>[2x]GPAAKSPENVYPVKTFGFAAKDSSGFFSPFNFSRRATGENDVQFKVLYCGTCNYDLEMSTNKFGMTKYPFVIGHEIVGVVTEIGSKVQKFKVGDKVGVGGFVGACEKCEMCVNGVENNCSKVESTDGHFGNNFGGCCNIMVVNEKYAVVWPENLPLHSGVPLLCAGITTYSPLRRYGLDKPGLNIGIAGLGGLGHLAIRFAKAFGAKVTLISSSVKKKREALEKFGVDSFLLNSNPEEMQGAYGTLDGIIDTMPVAHSIVPFLALLKPLGKLIILGVPEEPFEVPAPALLMGGKLIAGSAAGSMKETQEMIDFAAKHNIVADVEVIPIDYLNTAMERIKNSDVKYRFVIDVGNTLKSPSF

Crystal structures of THAS (here referred to as THAS1), a second representative THAS (Cr_021691, THAS2) and the structure of the promiscuous homologue (Cr_032583b, HYS) were solved and mutants revealed key residues that control the stereochemistry of the product profiles. The HYSs perform a single, chemically straightforward reduction reaction that immediately neutralizes the reactivity of strictosidine aglycone/cathenamine. The biological unit is an elongated homodimer, with each subunit divided into a substrate and cofactor-binding domain; the latter also being responsible for forming the dimer interface. The active site cavities of the HYSs are framed by helix α2, the catalytic zinc coordination sphere, and loops 1 and 2, with the NADP(H) co-substrate binding at the base of the active site.

Notably, one enzyme (Cr_032583b, HYS) produced a dramatically different product profile consisting of a mixture of ajmalicine/tetrahydroalstonine/mayumbine (55:27:15, at pH 6). HYS, which has a distinctly different product profile, was also crystallized to explore the structural basis behind this distinct stereochemical outcome. Structures were obtained for THAS1 and THAS2 with NADP+ bound (THAS1, 1.05 Å resolution; THAS2, 2.10 Å resolution) and in apo form (THAS1, 2.25 Å resolution; THAS2, 2.05 Å resolution), while HYS could only be crystallized in the apo form (2.25 Å resolution). The histidine residue in HYS loop 2 (His127) appears to be positioned appropriately to provide an alternative proton source for the opposite (‘top') face of the substrate, which could explain the appearance of ajmalicine in the product profile of HYS. Reactions with THAS1 and HYS performed at different pH conditions revealed that while changes in pH did not substantially impact the product profile of THAS1, HYS produced increased amounts of ajmalicine relative to tetrahydroalstonine at pH 6 compared with higher pH values. The increased level of ajmalicine in HYS at lower pH values is consistent with the pKa value of the histidine side chain and supports the role of this histidine in ajmalicine biosynthesis, though attributing pH dependence to specific residues must be approached with caution. While the THAS1 mutant containing the swaps displayed reduced activity rather than an altered product profile, the HYS mutant containing the shorter THAS1 loop 2 resulted in a product profile similar to that of THAS1. Therefore, we mutated this histidine to alanine or asparagine in HYS. Both of these mutants gave the same THAS-like profile, suggesting that His127 is required for producing the ajmalicine (R C20) stereochemistry. Interestingly, a non-proline cis-peptide is present in the THAS1-NADP+ and HYS apo structures.2-[(3-methylbenzyl)amino]ethanesulfonic acid | C10 H15 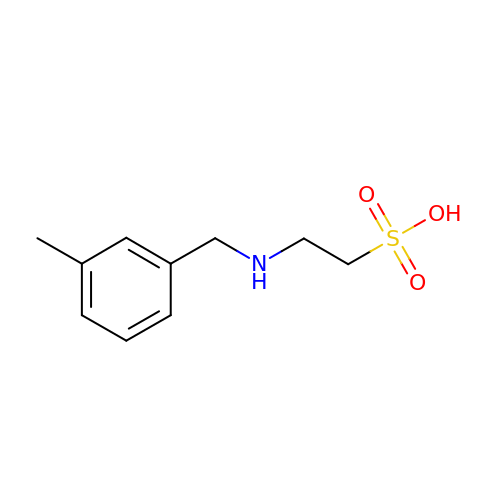N O3 S | KFWFDYYSPMOXBY-UHFFFAOYSA-N>VLGKPQTDPTLEWFLSHCHIHKYPSKSTLIHQGEKAETLYYIVKGSVAVLIKDEEGKEMILSYLNQGDFIGELGLFEEGQERSAWVRAKTACEVAEISYKKFRQLIQVNPDILMRLSAQMARRLQVTSEKVGNLAFLDVTGRIAQTLLNLAKQPDAMTHPDGM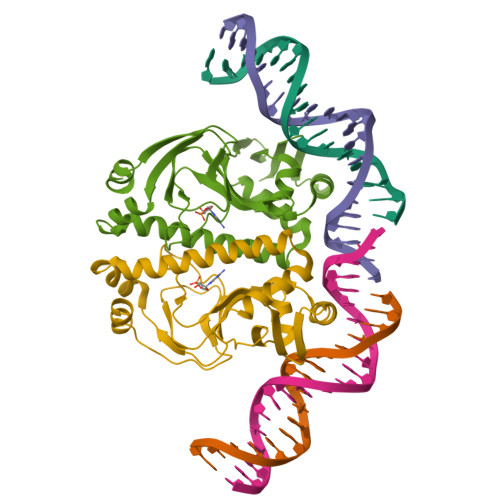QIKITRQEIGQIVGCSRETVGRILKMLEDQNLISAHGKTIVVYGTR[2x]> GSLDIAVYWGQSFDERSLEATCDSGNYAYVIIGFLNTFGGGQTPALDISGHSPKGLEPQIKHCQSKNVKVLLSIGGPAGPYSLDSRNDANDLAVYLHKNFLLPPAGTSESRPFGNAVLDGIDFHIEHGGPSQYQLLANILSSFRLSGSEFALTAAPQCVYPDPNLGTVINSATFDAIWVQFYNNPQCSYSASNASALMNAWKEWSMKARTDKVFLGFPAHPDAAG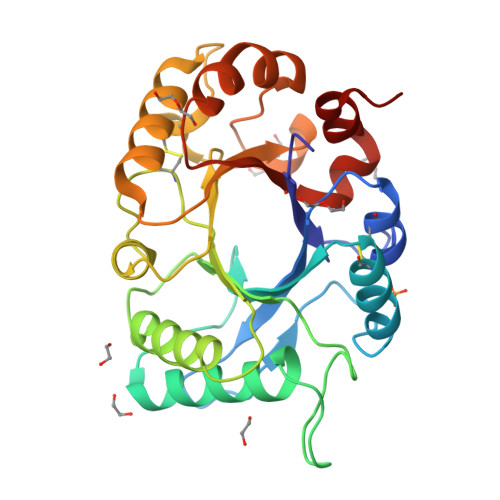SGYMPPTKVKFSVFPNAQDSTKFGGIMLWDSYWDTVSQFSNKILGKGV> MCSSINEGPYNSPTFGKSLSLKVDGGFNAVSINPSGRDIVLASRQGLYIIDLDDPFTPPRWLHHITPWQVADVQWSPHPAKPYWIVSTSNQKAIIWNLAKSSSNAIEFVLHGHSRAITDINFNPQHPDVLATCSVDTYVHAWDMRSPHRPFYSTSSWRSAASQVKWNYKDPNVLASSHGNDIFVWDLRKGSTPLCSLKGHVSSVNSIDFNRFKYSEIMSSSNDGTVKFWDYSKSTTESKRTVTTNFPIWRGRYLPFGEGYCIMPMVGGNNAVYLINLCDDDDSEQNKKTKLQPIYAFKGHSDRVIDFLWRSRHTCDGDYDDREFQLVTWSKDCDLKLWPISDSIYGKVNFDRGKRLEEKLPDYDYCSYNKEPENRENVQKNEFRRLRENFVTTSGLKKNKTNHITWLSGIRMNSATSQEDLFNETKIQNLGEEVSAIGHKFPKVVFEKISVSTRELCLTLNGPWSEENPDDYIFLRISINFPLNYPNKGDPPKFTIEENSNLTMSKRQEILSNLATIGQKYTDSNLYCLEPCIRFVLGEKVSLEDIEEGQEPLLNFDIADHIDFEELSSLDSSYSDSQNPENLSSQSDIESYKEALVFPDTSNQGLDFGRNLALDTTPVPNGCGSCWTATGELFCFFANEKKPEKKQNAIIKLSQKEAGVEKHPFKIEPQVLYDKEVDSSVITAADELKARPKRYVDTLGLGGGTNGDSRTYFDDETSSDDSFDSVADDWDDILRNDIIVRTKIPILRGNFKAFSSVHSESGKTVESTKKNKNLVISKNFSSLLSDRKELALEYLFMDATPEGFARNNALVAEKFDLDEISHCWQILSDMLIDQSDYDPYTTIWNNHPMGIKWFIKEAIVYFERQQNLQMLAMLCCVILSARRKKIPARYYGQELENMEGTIVFNDNESQNTSFWKGSDAFSTRSRSSTVTPNFYGNHLRGKNIHGGDNSSIRSDDHHARLRTHNTLNGSSKFTEPAQKQGSRAISSSPFHSRMPDIKVELLHDDIIEAYEQEDLLHLEVSDIPKFQTYIYQYSKLLFRWGLPLERVKILKVSTDFRSSYSSQGIPPNNNKKSPYNGVLTHWIENNEFGEEKFLARNCNYCDLRVTRSSFICGNCQHVLHSSCARIWWEIGDECPSGCGCNCPEMFDA;> MLSYFQGFVPIHTIFYSVFHPTEGSKIKYEFPPNNLKNHGINFNTFKNYIIPKPILCHKLITFKYGTYRIVCYPVTINSPIYARNFFSFNFVFVFPYDCETSPYEPAITRLGKMFKVLEEQNQLLSKSERDPVFFDLKVLENSTTTPSTAGPSSTPNPSSNTTPTHPTSEKDTKDMRSSRYSDLIKDLGLPQSAFSIQDLLMRIFQDLNNYSECLIPIDEGNAVDIKIFPLLRPPTTCVSLEDVPLSSVNLKKIIDVNWDPTMMSIVPYIDGLNSIAKISKLSNSDPGLVIECIRHLIYYKCVTLSDIFQFSNIYAPSSLIRNFLTDPLMASDCQSYVTFPEVSKISNLPLNKSLGSGDQDSPSFSVRRKSKSSSIPSNPDSRTTSFSSTSRVSQNSSLNSSFSSIYKDWRQSQTSCSSSNIHVINNRNRFLPTRSCLFDLYRSLSQGQTLKTWYESKYMILKENNIDIRRFITFGLEKRIIYRCYSFPVMINAGSREPKEMTPIITKDLVNNDKLLEKRNHNHLLSATGSRNTAQSGNLKPERPSKVSFEMQRVSSLATGKSTMPKLSDEEEGILEESIRNAETFDKICVLLSKPKLEVESYLNELGEFKVINS;> MDECLPNSCLLGVHLVISTHSGPQIVYHYPPSNTAFLTNNPTKHQHLYGNHANLNKNTSTNKEEKLFNSGSTKTASQIALNESAKSYNTAITPSMTNTNTNNVTLPPTRSHANTVGSQSSIPAATNGVGYRKTDIEDTSRTFQYQETESETSSSGLSDSELSTDYLDISSDSFSISSSLSSSSLSSSPSSSSSSSPPQDGLSRTNSSFQSTDSMSPTSPQMIMENDSISVAESYLDSGTNNKSRAASKRSQNFFHKLSTKKSTDSKTHSPVRKLKSKPSQSTKKGNKLLKNTSNETDGNAFTGSCSISSKKSLSSTGEHNQELRNSSLNDTPGQSPHHYHHRYHHYHKNAATSQRNSHTQYDVEEEDMEVSAMLQDGKISMNEIFFEEENFQDINKILEFDNDFVAEFCSPEREMCNTRFEFTVDNFCFLGLPIHVDSQGRWRKSKHKNKTRSKRSSSTTTNISRKKSIASKISSLSENTLKKVNSGE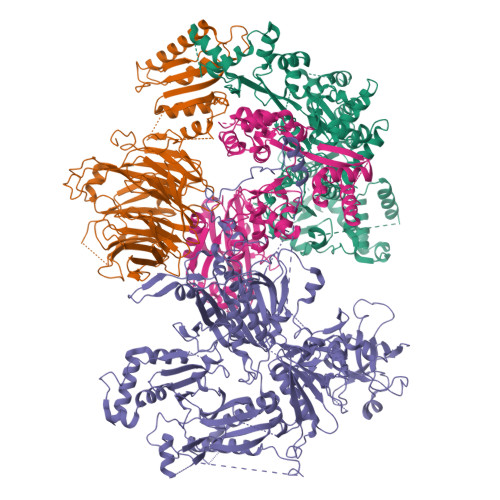ADTVYDSNIGHEASTDTPNLRINTDVSGNEFEREKEDLGKNMNMFHVCFVMNPHLIEYNKRIDDMYQFVVTRLSLLLRYVQSKTSYISSECHIILKEKERVLKHSKTYQSIRGAGNKGKYLYQRILAKSSLARALTECVDKIQRNEIACLEINDDKVISLQIPIQNEFEKMPNFKLQPVLRGSYLTSILNMKFLEKSSLRIESQNRQNDQAQFSDTNNNIYRFGNNINSTGHCGAANVDDGDDNESNYYCDDNDDLLNYALLLLDEPNNIISSLETFSYQDDIGTIILKHLVRNIQPNIPLRSYRYLITDLLDNPSSLDDLTTETNSLESSILRSCALHLMYWRHARIVIPLSSKYTYIVSPLAPIQGYTIDDYKSTSQNDGNVKKMDDRENNKSGSDRVPLIYQNSMLFRSKFPSLPSLPIFLSLLSTDKPQAYSNIIPSREHKPVYLNALAWLIQYGYVTQLLTFINIRVDKHIKMAVDEDLEKEGFRKTNTARRPSMDYKKTDKKLDDEDGQSRDANASEACSGKNEGMQSNDNNKDVDEKDNENDSRVDDRDDNEIAIADEEEILHFEYDDPEMQHDYTIILEPERATAIEKRWLYRCIYGQPSDIQILFNKLLKYFNGKVPMELVIIKEEISRHDLKKLLNALDKYLIEIHHW;> MFAKLHGKKQRPISSINSQTPRTSNTTHANSISLSSGNLIVGSNRNLRQKKEQFGSQQRASGRKLISNKENDDNVNNGGDNNYDNGERVHRHHIPGLKIKAYQAELGYHESRFSENLVMLNLVEFPDIKPGDLVELKTYHKNPSASNGDKKIYFIAKDFDGETKRRAKTSNVSILSGQLQTLLDLPSRSRIWIKLKPNKFDLQADVVEFNIKDCLLNRGDMWVLSSKLVDTCVFMDQRLAFLDSIRGTIKGIYRNGKKIVSGYIGEQTRIIFRSESARLIFLIQITDEMWNFEETGEQLFQKMVNSFFPKIFKKWKDVDTHHTITIAFAISMDLSDTSFKDLTPGESLKNSQDYFRIVVDQVSIIHWVDIMETLREEFMEIRKDLLNKQTDKGYSVANGRFSPVIKSNFLELVNFATTILTDPFKQLDLRHTTTHVMIISPGSGLFDVDYSLLRLTGKKLLSLEMTMDLICLSKAPLHIVPLFRYRDFENKLHHCVPLWLSVFFWNDHDKKSNSEWTPRCKIYDLQMMGITENELIREVDVEYLQLNKKVKSLSEFMNDYDKNAFEVKILCAGSNTKQSKKLNSKFDTVFENDVVVKARKIPATATTTHGNTKFIWRGPKVALPAIKDIQKPNVIPDLSIKTIEASFYDDCNTTNDKISTPTTSNNDNLEMNDSLVSVRSADNQNTSLALDSLKGLSKRNSLKDFTQRVITKFISNIDTSKNKKIKSTLLRDDVDNSPLGSNTPLPSSESKISGLKLQQKGLADENVISKRGNLIIKKNLSIFGLPSNEIMSGSPSSYLGSSHTRTSSKLSNMSDKAAFITEGQKSKHDDSNTYSLTQQLKHRISETWVDIKSPSIPVSSEFANELLPIRWKDVWPKYVARKYSKWRSFTTPAELPITISDFPSKDDFDRNFIFRNHSVTLNTDQEQYNQTYKDLLRDMIYMRLLTGFQICVGRQVEKIELSRESGESETVVNKYLDFNQNDAFKLYLMIDSEIHRITCSSSGIIDVERYLRKDEANLFDQVPSYIPLVKTRYESSFRDAMIDPLHVKRESLNWNQIDQVLAGYGDNLIDRKWHGFRAKYVVLPTDIPPNTYSMVINGKSETLNPEEIRVEGLRRLIGSITRSRLRTEKEKKGRKTKREEIQPEVMFYTGPLYNFINEQQTSLESSAINFKDSIFVNDNNLLNRNVELSKLAYQIQRGEDRITLVNRKWHWKKHEKCFVGSEMVNWLIRNFSDIDTREDAIKYGQKVMKEGLFVHVLNKHNFLDGHYFYQFSPEYVMDTNKLEKTNSHRSTLSDPKQMLRKASTGSSNDPSAMTPFSSVVPAISASNASVADAKEPSRPILMLSNSLVIDVDPAGKSSKQESCTVHYDRVHNPDHCFHIRLEWLTTTPKLIDDLVGNWSRLCERYGLKMIEIPWEELCTIPSVNPFHSFVEIKLAINPWEDPEFKDRELFAKSKFYYHVYLLKASGFLLDNRASKFLQNQDIEFDIMYSWGKPQFKYVQYIHHTGAYVAELRENGCLFLAPNNIYISRVNPGNIIGKIHSASSSSLDAQKVILNFKSTCLDYQKLRSIFLDAKEMWITGKIVED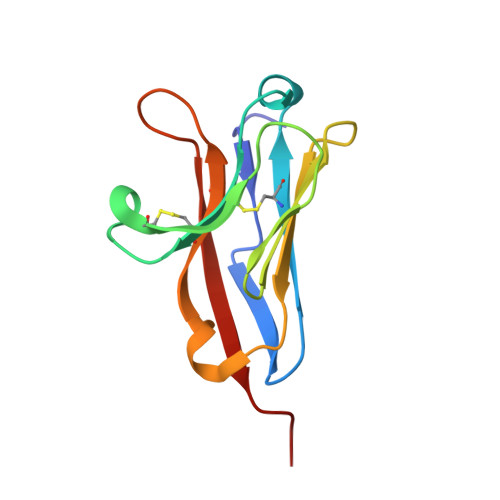> MEDPVTGPEEVSGQEQGSLTVQCRYTSGWKDYKKYWCQGVPQRSCKTLVETDASEQLVKKNRVSIRDNQRDFIFTVTMEDLRMSDAGIYWCGITKGGLDPMFKVTVNIGPVPT> MHHHHHHENLYFQSNAMRLDV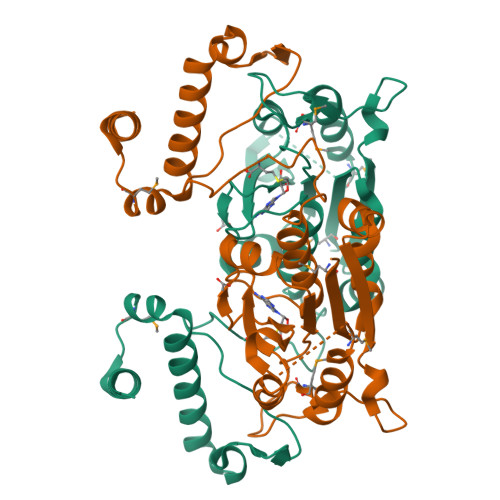ITIFPEYLDPLRHALLGKAIEKDLLSVGVHDLRLWAEDAHKSVDDSPFGGGPGMVMKPTVWGPALDDVATMSGKAHMGAQLDSARVHVDKPRHDELEGIQFAGYDAAEVAEADKPLLLVPTPAGAPFTQEDARAWSNEEHIVFACGRYEGIDQRVIEDAKKTYRVREVSIGDYVLIGGEVAVLVIAEAVVRLIPGVLGNTQSHQDDSFSDGLLEGPSYTKPREWRGLEVPEVLTSGNHAKIERWRREQSLKRTWEVRPELLDGMELDRHDQAYVEGLRRGNTSDNLN>GSPRLKFDVLENPNKGNKVNRSEQVNKSNNHAENPKPKEGVGTWVGKDIKVLTSKFGQADRVYPFRDGYKNYVFKDKNSYYIVSTKREEIVSVYATGEKVNVSPLKIGQHSAEIFNHTSINPEPSFKVDGKKYEFELSDEDLKTQTLIKYGDIYAQVYSDQQSKKVLSVRFLTKEMLADIEPYQLNSNSTSEEHNKRPVEQNPNQLISLYEVTNEMRKLKGLKPLKINSDLAHIASNNLYEATSNGSDSVEFTEDALRGQLDKNHVTYKTTAQNVGYAFNDVPTLIHSW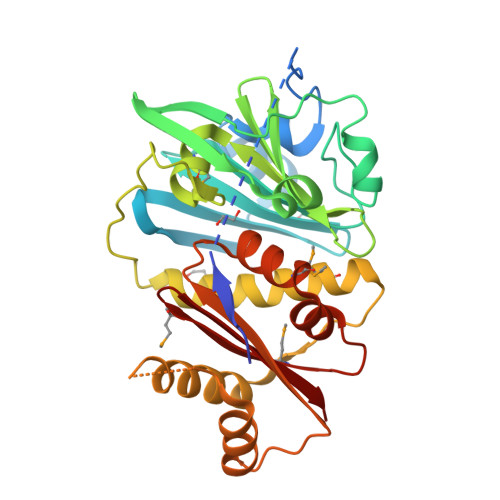MNSDIHRSRLLNSKYDEMGGDVMRDYYSLIFLEK[2x]> ADLGSHHHHHHGGMSLLSSIPMVSEQQHCIQHNHSSITFSLLTNKSD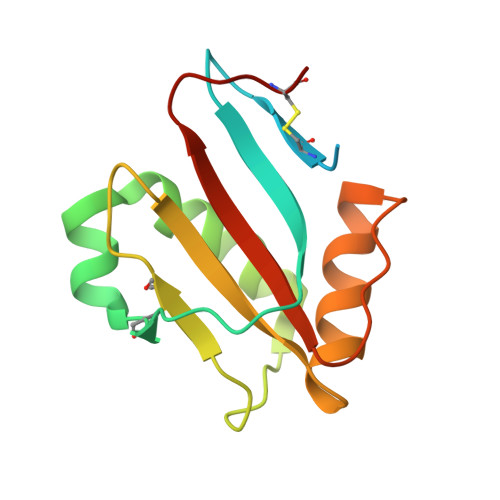LEKCNFTRLQAVDRVIFDLFREFHHRVGDFPVTSDLKCSHNTSYRVIEYEVTKESLPRLQEAVSTLFPDLHLSEDRFLQIQAHDDKNCTGLH3-(pyridin-3-yl)benzoic 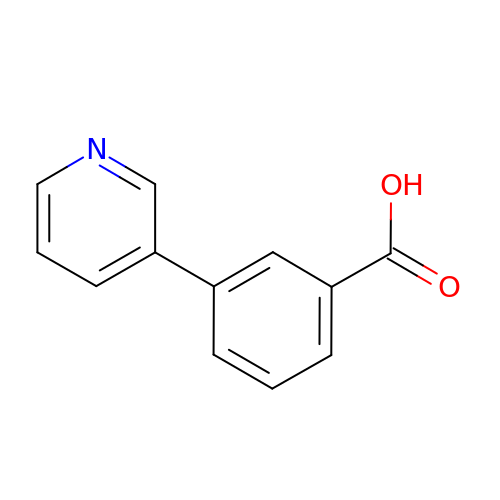acid | C12 H9 N O2 | PXASTGBSGPFLFJ-UHFFFAOYSA-N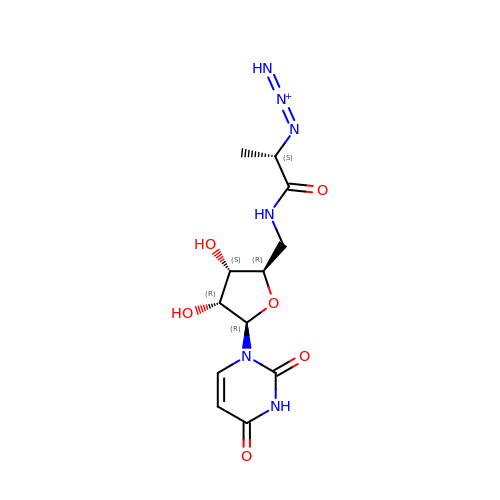5'-deoxy-5'-{[(2S)-2-(triaza-1,2-dien-2-ium-1-yl)propanoyl]amino}uridine | C12 H17 N6 O6 | BMVPLHCMGOWMGY-DANLAGSESA-O>KVLTIKSCNIHSGIGIRPHAQIELEYQGKIHKEISEGDGGYDAFMNALTKITNRLG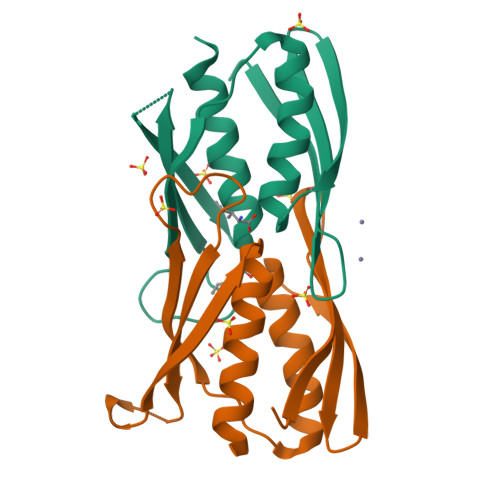ISIPKLIDYEVRIPPGGKTDALVETRITWNKSLDLEEDQTFKTMGVHPDQTVAAVHATEKMLNQILQPWQI[2x]> MDEEREKLKEKLKEVLRRAKEAKKKGDKEKLIELAYEAAALAAWIIHKDSNDDEIVELAKEALKLVLEAAKEAKKNGDKEKLIKLAYLAAAVAAWIIHTDGDDDEIVELAKEALKLVLEAAKEAKKNGDKE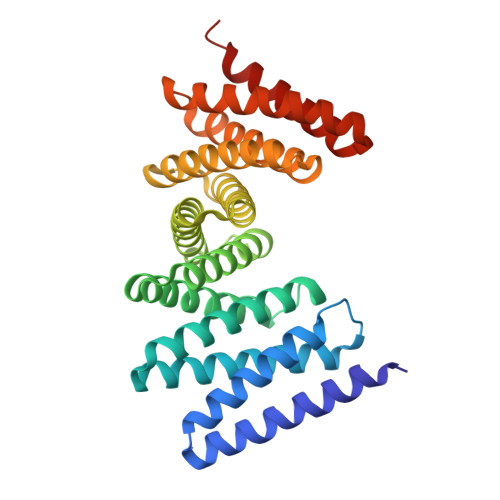KLIKLAYLAAAVAAWIITTDGDDDEIVELAKEALKLVLEAAKEAKKNGDKEKLIKLAYLAAAVAAWIIHTDGDDDEIVELAKEALKLVLEAAKEAKKNGDKEKLIKLAYLAAAVAAWIITTDGDDEEIVELAKEALKLVKEAAEEAEKQGDEELREKLRYLSEAVREWIERND> GAMERKTVLVIADLGGCPPHMFYKSAAEKYNLVSFIPRPFAITASHAALIEKYSVAVIKDKDYFKSLADFEHPDSIYWAHEDHNKPEEE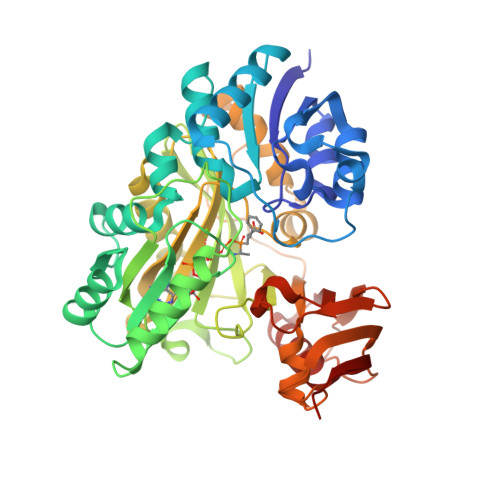VVEQIVKVAEMFGADAITTNNELFIAPMAKACERLGLRGAGVQAAENARDKNKMRDAFNKAGVKSIKNKRVTTLEDFRAALEEIGTPLILKPTYLASSIGVTLITDTETAEDEFNRVNDYLKSINVPKAVTFEAPFIAEEFLQGEYGDWYQTEGYSDYISIEGIMADGEYFPIAIHDKTPQIGFTETSHITPSILDEEAKKKIVEAAKKANEGLGLQNCATHTEIKLMKNREPGLIESAARFAGWNMIPNIKKVFGLDMAQLLLDVLCFGKDADLPDGLLDQEPYYVADCHLYPQHFKQNGQIPETAEDLVIEAIDIPDGLLKGDTEIVSFSAAAPGTSVDLTLFEAFNSIAAFELKGSNSQDVAESIRQIQQHAKLTAKYVLPV>MVRER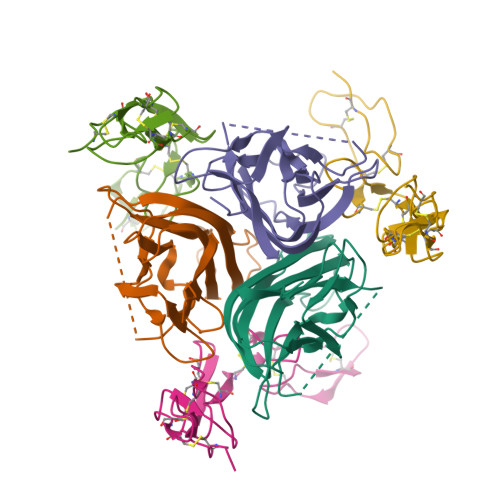GPQRVAAHITGTRGRSNTLSSPNSKNEKALGRKINSWESSRSGHSFLSNLHLRNGELVIHEKGFYYIYSQTYFRFQEEIKENTKNDKQMVQYIYKYTSYPDPILLMKSARNSCWSKDAEYGLYSIYQGGIFELKENDRIFVSVTNEHLIDMDHEASFFGAFLVG[3x];>[3x]HSPLGELCPPGSHRSERPGACNRCTEGVGYTNASNNLFACLPCTACKSDEEERSPCTTTRNTACQCKPGTFRNDNSAEMCRKCSTGCPRGMVKVKDCTPWSDIECVHK> SWA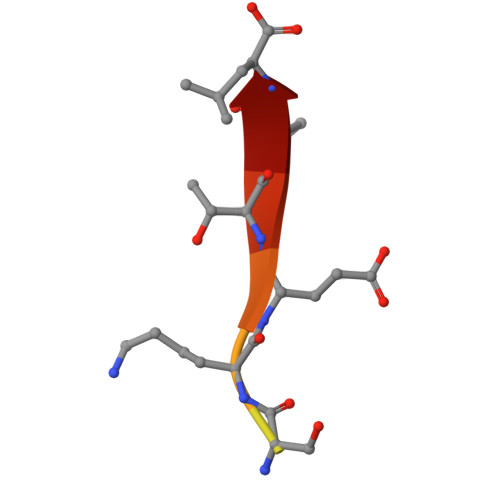RVSKETPL>SMSSQFIFEDVPQRNAATFNPEVGYVAFIGKYGQQLNFGVARVFFLNQKKAKMVLHKTAQPSVDLTFGGVKFTVVNNHFPQYVSNPVPDNAITLHRMSGYLARWIADTCKASVLKLAEASAQIVMPLAEVKGC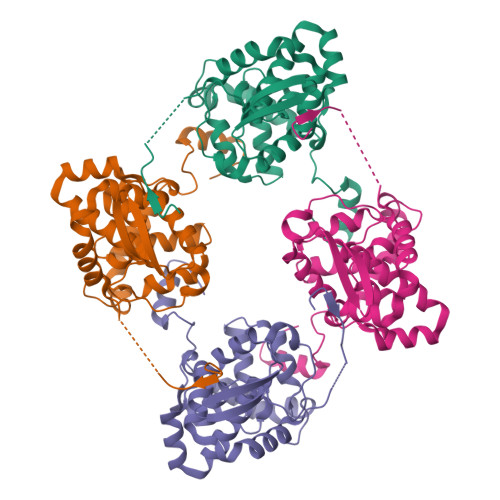TWADGYTMYLGFAPGAEMFLDAFDFYPLVIEMHRVLKDNMDVNFMKKVLRQRYGTMTAEEWMTQKITEIKAAFNSVGQLAWAKSGFSPAARTFLQQFGINI[4x]>MQKYALHAYPVMALMVATLTGCA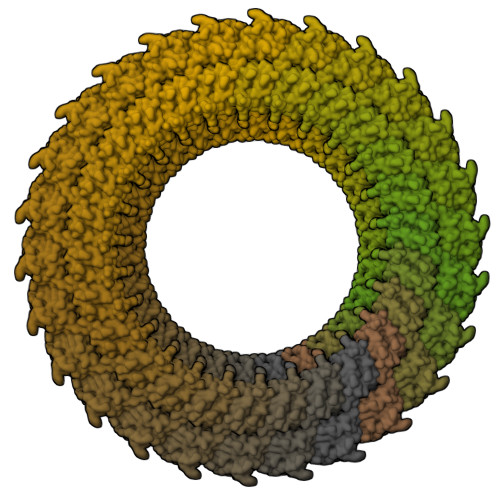WIPAKPLVQGATTAQPIPGPVPVANGSIFQSAQPINYGYQPLFEDRRPRNIGDTLTIVLQENVSASKSSSANASRDGKTSFGFDTVPRYLQGLFGNSRADMEASGGNSFNGKGGANASNTFSGTLTVTVDQVLANGNLHVVGEKQIAINQGTEFIRFSGVVNPRTISGSNSVPSTQVADARIEYVGNGYINEAQNMGWLQRFFLNLSPM[26x];>[26x]MFKALAGIVLALVATLAHAERIRDLTSVQGVRENSLIGYGLVVGLDGTGDQTTQTPFTTQTLNNMLSQLGITVPTGTNMQLKNVAAVMVTASYPPFARQGQTIDVVVSSMGNAKSLRGGTLLMTPLKGVDSQVYALAQGNILVGGAGASAGGSSVQVNQLNGGRITNGAIIERELPTQFGAGNTINLQLNDEDFTMAQQITDAINRARGYGSATALDARTVQVRVPSGNSSQVRFLADIQNMEVNVTPQDAKVVINSRTGSVVMNREVTLDSCAVAQGNLSVTVNRQLNVNQPNTPFGGGQTVVTPQTQIDLRQSGGSLQSVRSSANLNSVVRALNALGATPMDLMSILQSMQSAGCLRAKLEII> GGCGGCAGGUGCUCCCGACCCUGCGGUCGGGAGUUAAAAGGGAAGCCGGUGCAAGUCCGGCACGGUCCCGC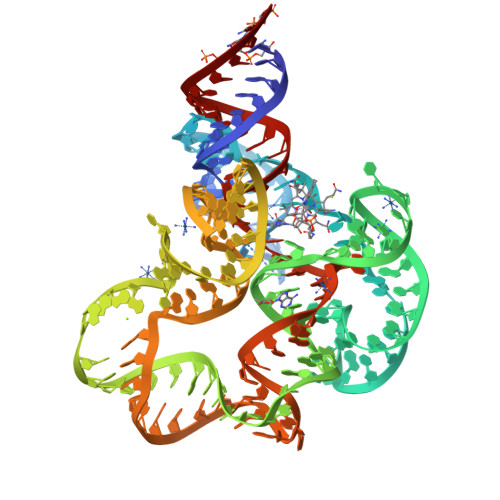CACUGUGACGGGGAGUCGCCCCUCGGGAUGUGCCACUGGCCCGAAGGCCGGGAAGGCGGAGGGGCGGCGAGGAUCCGGAGUCAGGAAACCUGCCUGCCGUC>[7x]GPE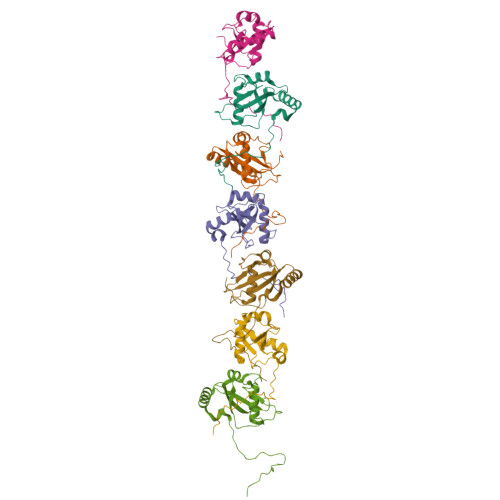ESWEDDIAGQRTFPEDPNYPVMKSTFKSEYPFEKRKAESERIADRFPNRIPVICEKAEKSDIPEIDKRKYLVPADLTVGQFVYVIRKRIMLPPEKAIFIFVNDTLPPTAALMSAIYQEHKDKDGFLYVTYSGENTFG4-[2-(2-methylpropyl)-1,3-thiazol-4-yl]-~{N}-[3,3,3-tris(fluoranyl)propyl]benzamide 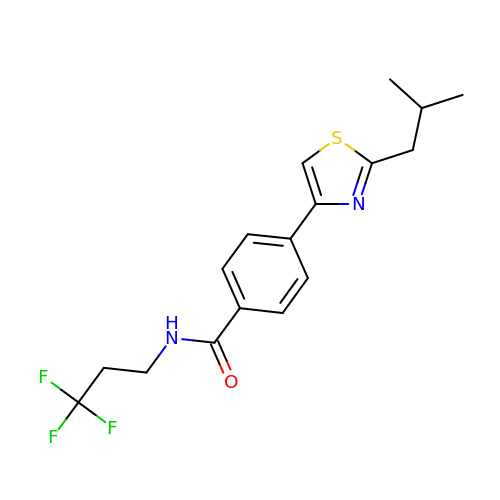| C17 H19 F3 N2 O S | UBQMCDSKFNKYKI-UHFFFAOYSA-N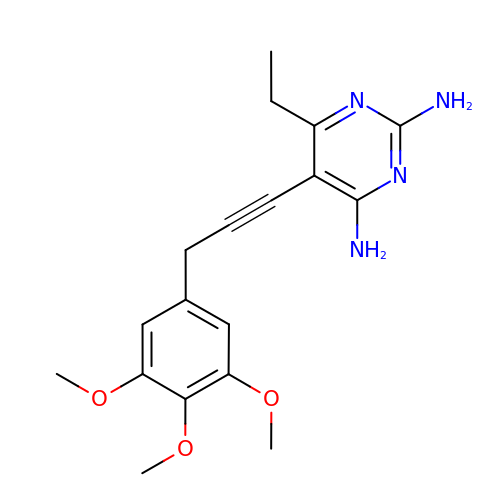6-ethyl-5-[3-(3,4,5-trimethoxyphenyl)prop-1-yn-1-yl]pyrimidine-2,4-diamine | C18 H22 N4 O3 | VPNXKXUNASBBLU-UHFFFAOYSA-N>GHMSGVLQISFPAGIAAIRNNSSLR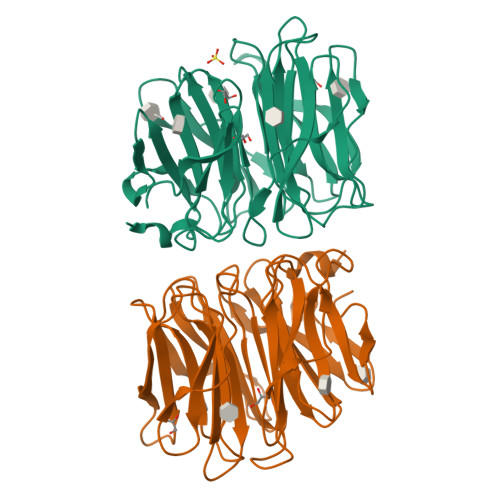VYEAALDGGVREAQYEGRWAGGKPDNVIATGKIGTPIAATSVGFQYIRVYYVGADNKAREACWDGKGWYTGAFVKDVAPYSSIGAVFLGKNIVVRVYTQNHDNTIQEWVWDSPSTGWTAGANFGAALPGTAIAATSWGAGPYHIRVYFQDTNRNVIESGWDGSGWYTGGLKISNQSPRASLGATSWGESGSSLGIRLYYATQDNLIKEKAWDGGGGWYDGGFQQRSIPGSRVAAIPLPVLRVYLQNGTEVSGITEYAWNSGWVVGQAVLPPA[2x]1,5-anhydro-2-deoxy-2-(ethanethioylamino)-D-arabino-hex-1-enitol | 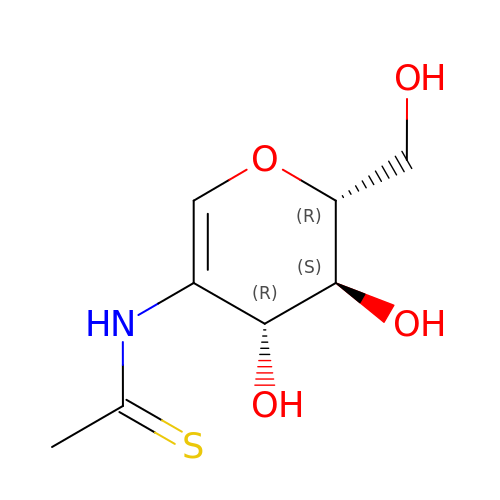C8 H13 N O4 S | VWPHMQQBRGEPGS-BWZBUEFSSA-N>[2x]RAPAPATPHAPDSPAPNSPTLTRPPE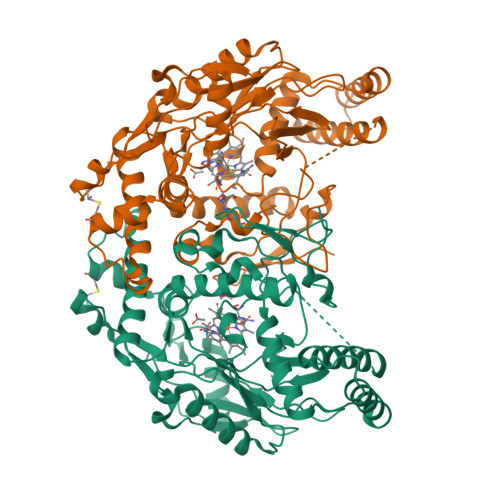GPKFPRVKNWELGSITYDTLCAQSQQDGPCTPRRCLGSLVLPRKLQTRPSPGPPPAEQLLSQARDFINQYYSSIKRSGSQAHEERLQEVEAEVASTGTYHLRESELVFGAKQAWRNAPRCVGRIQWGKLQVFDARDCSSAQEMFTYICNHIKYATNRGNLRSAITVFPQRAPGRGDFRIWNSQLVRYAGYRQQDGSVRGDPANVEITELCIQHGWTPGNGRFDVLPLLLQAPDEAPELFVLPPELVLEVPLEHPTLEWFAALGLRWYALPAVSNMLLEIGGLEFSAAPFSGWYMSTEIGTRNLCDPHRYNILEDVAVCMDLDTRTTSSLWKDKAAVEINLAVLHSFQLAKVTIVDHHAATVSFMKHLDNEQKARGGCPADWAWIVPPISGSLTPVFHQEMVNYILSPAFRYQPDPW>[3x]XRMKQIEDKIEEIESKQK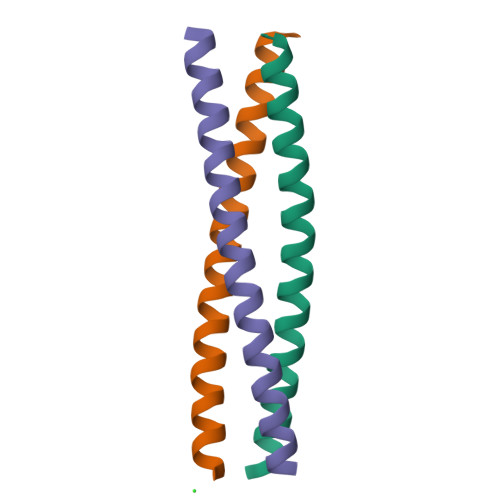KIENEIARIKKLLQLTVWGIKQLQARIL N-hydroxy-N~2~-{[3-(methoxymethyl)phenyl]sulfonyl}-N~2~-(2-methylpropyl)-D-valinamide 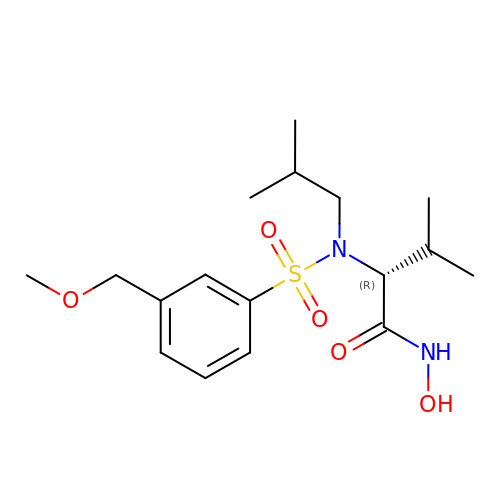| C17 H28 N2 O5 S | FSBJQCWNYNVFOV-MRXNPFEDSA-N>MMELIRIAMKKDLENDNSLMNKWATVAGLKNPNPLYDFLNHDGKTFNEFSSIVNIVKSQYPDREYELMKDYCLNLDVKTKAARSALEYADANMFFEIEDVLIDSMISCSNMKSKEYGKVYKIHRELSNSVITEFEAVKRLGKLNIKTPEMNSFSRLLLLYHYLSTGNFSPMAQLIKQIDLSEISENMYIRNTYQTRVHVLMSNIKLNENSLEECREYSKKALESTNILRFQVFSYLTIGNSLLFSNYELAQENFLKGLSISVQNENYNMIFQQALCFLNNVWRKENKWINFESDSIMDLQEQAHCFINFNENSKAKEVLDKLDLLVHNDNELAMHYYLKGRLEQNKACFYSSIEYFKKSNDKFLIRLPLLELQKMGENQKLLELLLLLEHH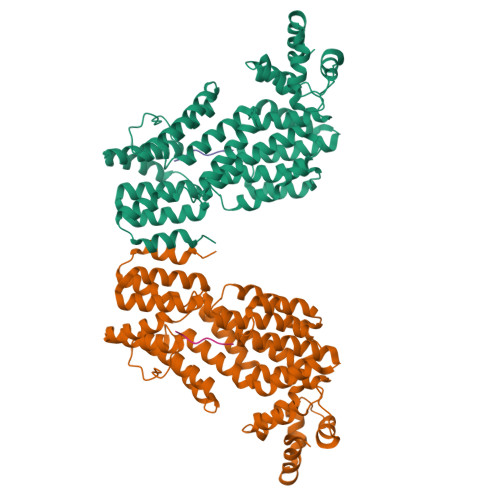HHHH[2x];>GMPRGA[2x]> MSVGLIAPLASPIQESRANTNIENIGDGAEVIKRTEDVSSKKWGVTQNVQFDFVKDKKYNKDALIVKMQGFINSRTSFSDVKGSGYELTKRMIWPFQYNIGLTTKDPNVSLINYLPKNKIETTDVGQTLGYNIGGNFQSAPSIGGNGSFNYSKTISYTQKSYVSEVDKQNSKSVKWGVKANEFVTPDGKKSAHDRYLFVQSPNGPTGSAREYFAPDNQLPPLVQSGFNPSFITTLSHEKGSSDTSEFEISYGRNLDITYATLFPRTGIYAERKHNAFVNRNFVVRYEVNWKTHEIKVKGHNKHHHHHH;> XDYDYG

Staphylococcus aureus (SA) leukocidin ED (LukED) belongs to a family of bicomponent pore forming toxins that play important roles in SA immune evasion and nutrient acquisition. LukED targets specific G protein-coupled chemokine receptors to lyse human erythrocytes (red blood cells) and leukocytes (white blood cells). Each leukotoxin is made up of two subunits of approximately 30 kDa: a host cell targeting S-component (HlgA, HlgC, LukE, lukS-PV, and LukA/G), and a polymerization F- component (HlgB, LukD, lukF-PV, and LukB/H), which can bind the plasma membrane through highly conserved phosphocholine binding sites. Each toxin is composed of two domains: a central β sandwich called the CAP domain and involved in inter-protomer interactions, and a RIM domain which contains several divergent loops driving host cell specificity.

Although CCR2 is normally an in vivo target of HlgA rather than LukE, Tam and coworkers have shown that cells expressing WT CCR5 or a CCR5 chimera harbouring the CCR2 N-terminal region display the same susceptibility to LukED intoxication. We found that sTyr26 and sTyr28 of CCR2 respectively bind to site 1 and site 2 through the same interactions observed in the pCS and ACKR1 peptide-bound structures. Two alternate conformations were clearly visible for sTyr26, differing by a rotation of approximately 90° of the phenyl ring. However, residual electron density was still present after model building and suggested the existence of a third alternate conformation of sTyr26, with its sulfate group interacting at site 2. This third alternate conformation clashes with the sulfate group of sTyr28, suggesting the existence of a minor population of molecules in which sTyr28 unbinds while sTyr26 flips its sidechain to the second site. Our work demonstrates that site 1 is used to bind ACKR1 sTyr 41, CCR2 sTyr 26, and CCR5 sTyr 10, while site 2 can accommodate an additional downstream sulfotyrosine such as CCR5 sTyr 14 or 15, or CCR2 sTyr 28. Site 2 is only conserved in LukE and HlgA, and likely confers to these toxins the ability to bind the second sTyr of the motif in the N-termini of CCR2, CCR5, and CXCR2.>[3x]MDFLSNFLTDFVGQLQSPTLAFLIGGMVIAALGTQLVIPEAISTIIVFMLLTKIGLTGGMAIRNSNLTEMLLPVAFSVILGILIVFIARFTLAKLPNVRTVDALATGGLFGAVSGSTMAAALTTLEESKISYEAWAGALYPFMDIPALVTAIVVANIYLNKRKRKSAAASIEESFSKQPVAAGDYGDQTDYPRTRQEYLSQQEPEDNRVKIWPIIEESLQGPALSAMLLGLALGIFTKPESVYEGFYDPLFRGLLSILMLIMGMEAWSRIGELRKVAQWYVVYSLIAPIVHGFIAFGLGMIAHYATGFSLGGVVVLAVIAASSSDISGPPTLRAGIPSANPSAYIGSSTAIGTPIAIGVCIPLFIGLAQTLGAG;>MAKPANKLVIVTEKILLKKIAKIIDESGAKGYTVMNTGGKGSRNVRSSGQPNTSDIEANIKFEILTETREMAEEIADRVAVKYFNDYAGIIYICSAEVLYGHTFCGPEGC[3x]

SbtA, which is ubiquitous in cyanobacteria, is an inducible high-affinity sodium-dependent HCO3– symporter within the TC.2.A.83 family of Na+/solute symporters. The sbtB gene from the sbtA–sbtB operon encodes a PII-like signaling protein that senses the intracellular level of the secondary messenger cAMP that correlates with high Ci conditions, versus AMP at low Ci conditions, thus functioning as a Ci sensor in cyanobacteria. The tightly packed trimeric structure of SbtA is exclusively stabilized by the gate domains at the center, with a threefold axis perpendicular to the membrane plane. In summary, this study provides structural insights into the cyanobacterial high-affinity HCO3– transporter SbtA, which exhibits a new architecture of Na+/solute symporters and its fine interaction pattern with a PII-like protein SbtB.

To elucidate the fine interaction mode between SbtA and SbtB, we purified the SbtA–SbtB complex in the presence of AMP and solved its 3.15 Å cryo-EM structure. The SbtB trimer is associated with the intracellular face of the SbtA trimer, sharing an overlapped threefold axis. Similar to the previously reported PII and PII-like structures, SbtB also adopts a trimeric structure, each subunit of which shows a canonical PII ferredoxin-like fold with a well-structured T-loop. In addition, an AMP molecule binds to the nucleotide-binding cleft between each pair of neighboring SbtB subunits. In the complex, the core structure of SbtB does not directly interact with the intracellular surface of SbtA. Instead, the structured T-loop of SbtB, which extends ~20 Å from the core structure of SbtB, is inserted into the inter-domain cleft of the corresponding SbtA subunit, yielding an interface area of ~740 Å2. Similar to the complex structure of AmtB–GlnK, in which the T-loop of PII protein GlnK inserts deeply into the cytoplasmic pore exit of the ammonia channel AmtB11, the SbtA–SbtB structure showed that SbtB T-loop partially blocks the substrate tunnel exit of SbtA, indicating that SbtB might attenuate the transport activity of SbtA under certain physiological conditions. At the peripheral side of TM crossover within the center of SbtA core domain in the SbtA–SbtB complex, there is a clear cryo-EM density most likely corresponding to a sodium ion, given SbtA is a Na+-dependent transporter. In each subunit, the Na+ forms five coordinate bonds with the main-chain oxygens of residues Phe110, Gly111, and Ala112 from TM4a and Ala320 and Ser322 from TM9a. As a result, the two domains of SbtA in SbtB-bound form are relatively separated from each other, yielding an inward-open conformation.> MSDFLNQYLLYLIKQYYEKPKANAEAQLLISTWETYADFIANFGNNFDIDNAEGEVLDLIGRILDLSRQVNDVIPASFFGFSENPLAKGFTSLENPLRVSAPFFKLTSKVYTDYQLTDTQYRKFLKVKAAKNICSPYLASDEKISLQQVVFDAFDGRAYVVDGKDQTLRLYVSPSIDDDELRLLINL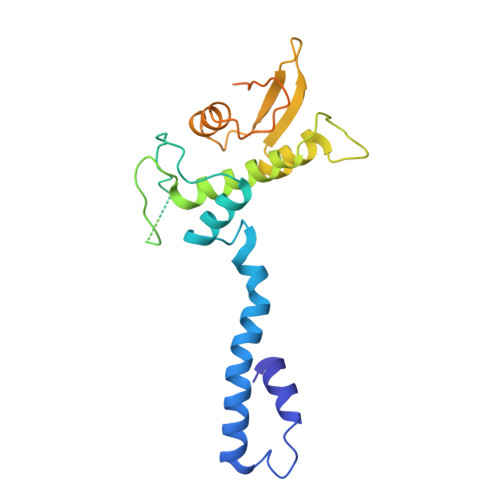DILPRPITFRYIIYGNAEPGVTFGFSNNPGSKSFGSLNNPSRQENGGVFARFYNG The CysN polypeptide also contains a C-terminal APS (adenosine-5’-phosphosulfate) kinase domain (CysC), which exists as a separate enzyme in other bacteria and plants. Alternatively, APS can be phosphorylated at the 3′-position by APS kinase (CysC) to generate 3′-phosphoadenosine 5′-phosphosulfate (PAPS), a substrate for sulfotransferases that catalyze the transfer of the sulfate group onto a variety of metabolites. The structure of CysC is characterized by the canonical α/β-purine nucleotide binding fold, consisting of a five-stranded parallel β-sheet which is flanked on both sides by two α-helices. Structural features typical of APS kinases of this fold family, including the P-loop required for ATP binding (residues 452–458 in CysC), the conserved LDGD motif (residues 477–480) and the lid region (residues 552–581) above the P-loop which closes upon substrate binding, are also found in CysC.

The structure of CysC with the non-hydrolyzable ATP analogue AMP-PNP, Mg2+, and APS bound in the active site provides a view of the Michaelis complex in the reaction sequence. The bound ligands AMP-PNP and APS are well defined in electron density and their interactions with CysC are, with the exception of the γ-phosphate group of AMP-PNP, essentially identical to those observed in the CysC•ADP•APS complex. The γ-phosphate extends from the ADP moiety towards the ribose group of APS, and the phosphorous atom is about 3.4 Å away from the 3’ hydroxyl oxygen, the acceptor of the phosphoryl group. An important contribution to the binding of AMP-PNP is the Mg2+ ion that is bound in octahedral coordination geometry in the active site. The ligand sphere of this ion consists of one oxygen atom each from the β- and γ-phosphate groups, the side chain oxygen of Ser457 and three water molecules (metal-ligand distances 2.0–2.2 Å). In the structure of the CysC•AMP-PNP•APS complex, helix α5 is shifted by about 2.2 Å closer to the nucleotide binding site compared to the structure of the CysC•ADP complex. The side chain of Asp478 forms a hydrogen bond to a water molecule that is ligand of the Mg2+ ion. The γ-phosphate group of the ATP analogue and the 3’ hydroxyl group of APS accepting the phosphate are well aligned with a distance of 3.4 Å between the phosphorous and the hydroxyl oxygen atom. In the transition state an increase of negative charge occurs at the γ-phosphate and the side chain of the conserved residue Lys562 is perfectly positioned to facilitate catalysis by stabilizing this charge as it is located between the γ-phosphate and the acceptor oxygen atom of the 3’ hydroxyl group of APS. In addition the conserved side chain of Asp480, close to the 3’ hydroxyl group of the acceptor substrate APS, could act as a catalytic base in deprotonation of the O3’ hydroxyl group.

>[2x]PPRGKTVWFTGLSGSGKSSVAMLVERKLLEKGISAYVLDGDNLRHGLNADLGFSMADRAENLRRLSHVATLLADCGHLVLVPAISPLAEHRALARKVHADAGIDFFEVFCDTPLQDCERRDPKGLYAKARAGEITHFTGIDSPYQRPKNPDLRLTPDRSIDEQAQEVIDLLES> MLQINAFKLVRATPFLLKRTGKPADTPDYKQVYLPYDAAPTERELERERRRFKQAYHGRMEHRKLVEVKEVPLNVYTYGKEGMSLPIAIFKDQKDPVIGPEWTYPGIYENKIAAQHWYTEELFDKESKEAFESPWQQQILDNQVKRRMAKVMFRMRQVNMKAV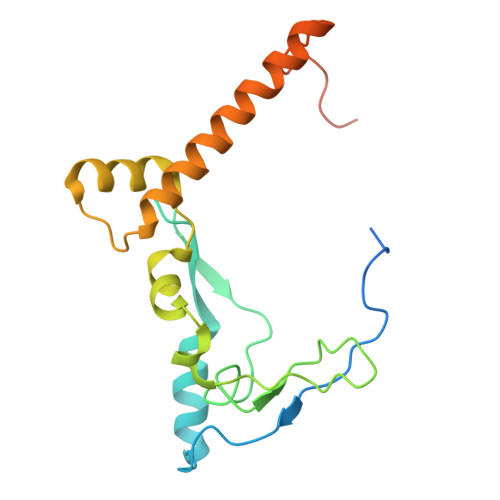DLFQKERGSSRRSGGAGEKGKDGGGKK The mRubyFT is a monomeric genetically encoded fluorescent timer based on the mRuby2 fluorescent protein, which is characterized by the complete maturation of the blue form with the subsequent conversion to the red one. It has higher brightness in mammalian cells and higher photostability compared with other fluorescent timers. Blue-to-red fluorescent timers (FTs) change their fluorescence color from blue to red during maturation. Monomeric blue-to-red fluorescent timers Fast-FT, mRubyFT and mTagFT have been developed from the mCherry, mRuby2 and TagRFP red fluorescent proteins, respectively, and the corresponding mechanism of timer maturation with the formation of a red chromophore through its blue form has been proposed.

For this purpose, we constructed the S148I point mutant of the mRubyFT (here and after—mRubyFTS148I), which stabilizes the timer in its blue state over time. The crystal structure of mRubyFTS148I was elucidated using an X-ray crystallography method at 1.8 Å resolution. There is one protein molecule per asymmetric unit, and contact analysis revealed that the protein is a monomer in the crystal. The chromophore positioned on the central helix of the barrel is formed by 68LYG70 amino acids. The chromophore is covalently bound to the neighboring F67 and S71 residues. Its imidazolidinone moiety is restricted on one side by the carboxyl oxygen of T65 and is additionally fixed by hydrogen bonds with R72, R97 and E220. The chromophore has a clear electron density except for its phenolic moiety, where density is poor. In this conformation, the phenyl oxygen of the chromophore is directly hydrogen bound to the side chain of T163 as well as to E150 and T181 via a solvent water molecule. At the same time, the poor electron density of the phenyl moiety suggests that it could be flexible as the oxidation of the methine bridge did not occur. Moreover, compared to the parental protein mRuby (corresponding residue H148), in mRubyFTS148I, isoleucine is shifted 1.3 Å closer (distance between Cα-atoms of corresponding residues) to the chromophore. This shift in the orientation of the I148 side chain hampers the rotation of the phenolic moiety of the chromophore to a cis conformation and restricts it from being coplanar with the imidazolidinone moiety. The absorption/excitation/emission band maxima at 407/410/460 nm are within a 3 nm difference from the blue form of the mRubyFT timer, indicating that the S148I substitution practically did not affect the photophysical properties of the blue chromophore but blocked the transition into the red form.

> GHMRSMVSKGEELIKENMRMKVVMEGSVNGHQFKCTGEGEGNPYMGTQTMRIKVIEGGPLPFAFDILATSFLYGSRTFIKYPKGIPDFFKQSFPEGFTWERVTRYEDGGVVTVMQDTSLEDGCLVYHVQVRGVDFPSNGPVMQKKTKGWEPITEMMYPADGGLRGYTHMALKVDGGGHLSCSFVTTYRSKKTVGNIKMPGIHAVDHRLERLEESDNEMFVVLREHSVAKFAGRGGMDELYK>[3x]VEDEEHIDLPPGFRFHPT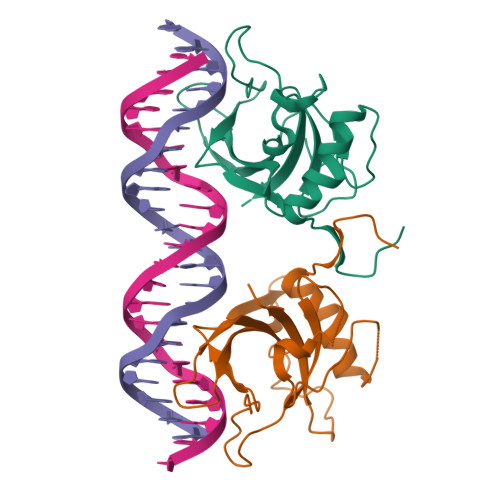DEELITHYLKPKVFNTFFSATAIGEVDLNKIEPWDLPWKAKMGEKEWYFFCVRDRKYPTGLRTNRATEAGYWKATGKDKEIFKGKSLVGMKKTLVFYKGRAPKGVKTNWVMHEYRLEGKYCIENLPQTAKNEWVICRVFQK>[2x]MNTISSLETTDLPAAYHIEQRAHAFPWSEKTFASNQGERYLNFQLTQNGKMAAFAITQVVLDE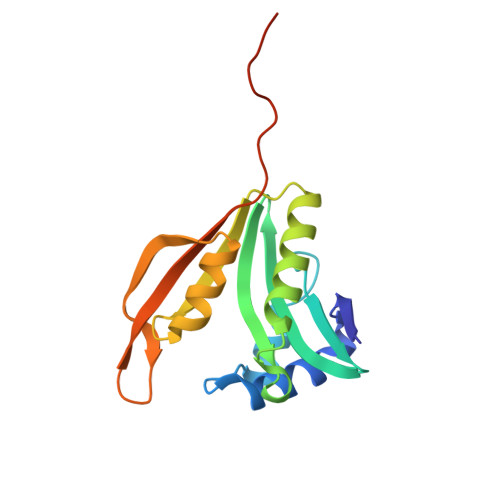ATLFNIAVDPDYQRQGLGRALLEHLIDELEKRGVATLWLEVRASNAAAIALYESLGFNEATIRRNYYPTTDGREDAIIMALPISMAGENLYFQSAGHHHHHH>[5x]GASQFFKDNCNRTTASLVEGVELTKYISDINNNT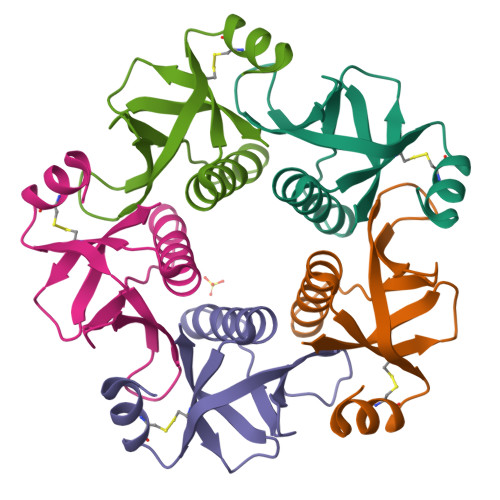DGMYVVSSTGGVWRISRAKDYPDNVMTAEMRKIAMAAVLAGMRVNMCASPASSPNVIWAIELEA N-[(4-amino-2-methylpyrimidin-5-yl)methyl]formamide 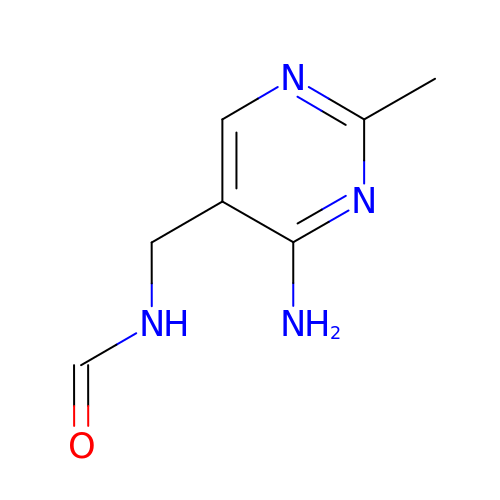| C7 H10 N4 O | PVWNFAGYFUUDRC-UHFFFAOYSA-N>MTSAEMTSPNNNSEHQAIAKMRTMIEGFDDISHGGLPIGRSTLVSGTSGTGKTLFSIQFLYNGIIEFDEPGVFVTFEETPQDIIKNARSFGWDLAKLVDEGKLFILDASPDPEGQEVVGGFDLSALIERINYAIQKYRARRVSIDSVTSVFQQYDASSVVRRELFRLVARLKQIGATTVMTTERIEEYGPIARYGVEEFVSDNVVILRNVLEGERRRRTLEILKLRGTSHMKGEYPFTITDHGINIFPLGAMRLTQRSSNVRVSSGVVRLDEMCGGGFFKDSIILATGATGTGKTLLVSRFVENACANKERAILFAYAESRAQLLRNAYSWGMDFEEMERQNLLKIVCAYPESAGLEDHLQIIKSEINDFKPARIAIDSL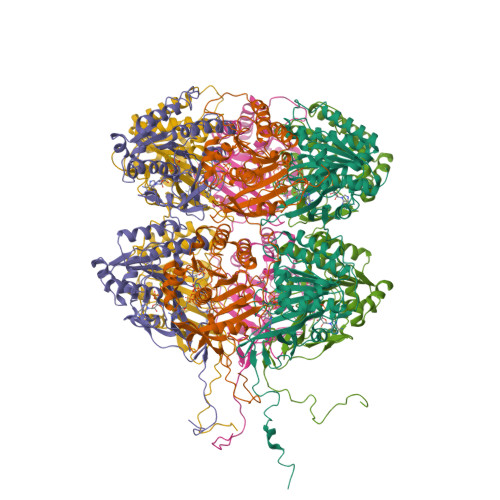SALARGVSNNAFRQFVIGVTGYAKQEEITGLFTNTSDQFMGAHSITDSHISTITDTIILLQYVEIRGEMSRAINVFKMRGSWHDKAIREFMISDKGPDIKDSFRNFERIISGSPTRITVDEKSELSRIVRGVQEKGPES[6x]>MSHPKQVGQYKLGKLLIEGKTKQVFDVPDQPGYCLLLNKDRITAGDGVKAHDLEGKAAISNQTNAKVFEILKSAGIKTAFVKIASETAFLSKKCEMIPIEWVTRRLATGSFLKRNPGVPEGFRFTPPKQETFFKDDANHDPQWSEEQIISAKFNYNGLLIGRDEVDYMRKATILIFEILEKAWALRDCALIDMKIEFGVDTEGSIVLADVIDSDSWRLWPSGDKRLMVDKQVYRNLTTVTAADLDTVKRNFAWVKDQLDFLKPTIHHKVVVFMGSPADQEHCQKIAKAARELGLDVDLRVTSAHKATEETLRIMQQYEDTHGALVFIAVAGRSNGLGPVLSGNTSYPVINCPPPSDKLVQDIWSSLSVPSGLGCATVIYPDSAALMAAQIIGLQDYLVWGRLRSKQLDMAHSLRQADKKL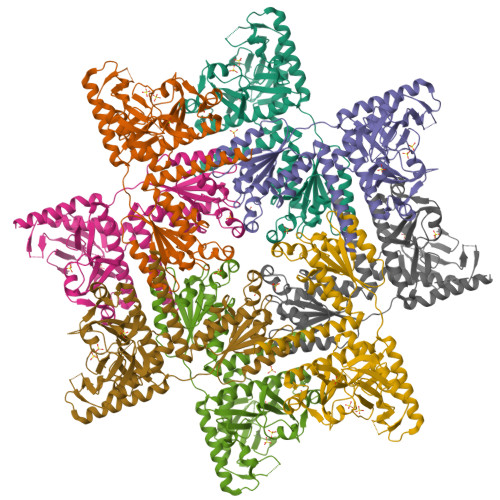RNQTA[4x]> MGSSHHHHHHSQDPNSMTTLTRQDLNFGQVVADVLCE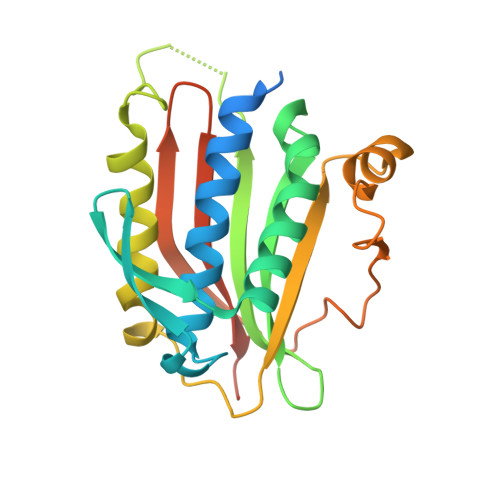FLEVAVHLILYVREVYPVGIFQKRKKYNVPVQMSCHPELNQYIQDTLHCVKPLLEKNDVEKVVVVILDKEHRPVEKFVFEITQPPLLSISSDSLLSHVEQLLAAFILKISVCDAVLDHNPPGCTFTVLVHTREAATRNMEKIQVIKDFPWILADEQDVHMHDPRLIPLKTMTSDILKMQLYVEERAHKGSGSGSGSGSGSH(4S,5E,8S,9E,11S,13E,15E,18R)-4-hydroxy-8-methoxy-9,11-dimethyl-18-[(1Z,4E)-2-methylhexa-1,4-dien-1-yl]oxacyclooctadeca-5,9,13,15-tetraen-2-one 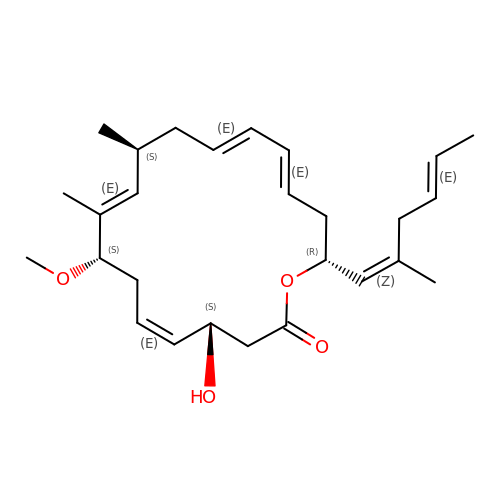| C27 H40 O4 | DVYYXLNVAXSASA-BEVCVMOBSA-N> SSNSCTTEDRREMQLMWANVWSAQFTGRR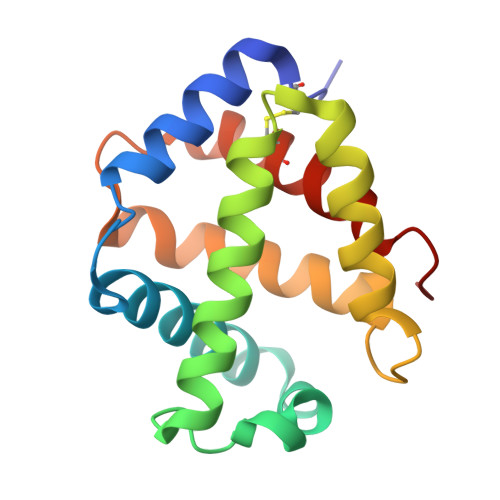LAIAQAVFKDLFAHVPDAVGLFDRVHGTEIDSSEFKAHCIRVVNGLDSAIGLLSDPSTLNEQLSHLATQHQERAGVTKGGFSAIAQSFLRVMPQVASCFNPDAWSRCFNRITNGMTEGLAE N~2~-[3-(2-hydroxyethoxy)propanoyl]-N-phenyl-N~6~-tetradecanethioyl-L-lysinamide | C31 H53 N3 O4 S | 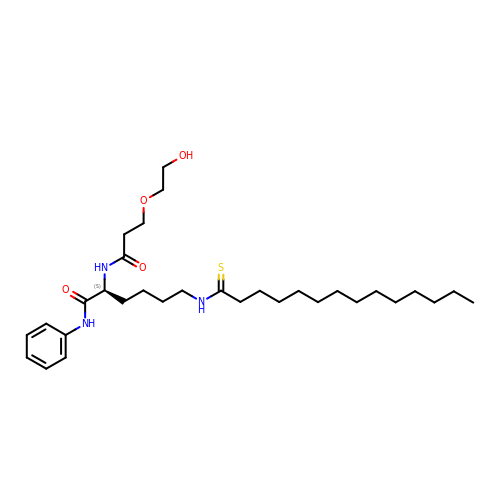IGGXAEJVAQDTLQ-NDEPHWFRSA-N> MQVHLTHFELEGLRCLVDKLESLPLHKKCVPTGIEDEDALIADVKILLEELASSDPKLALTGVP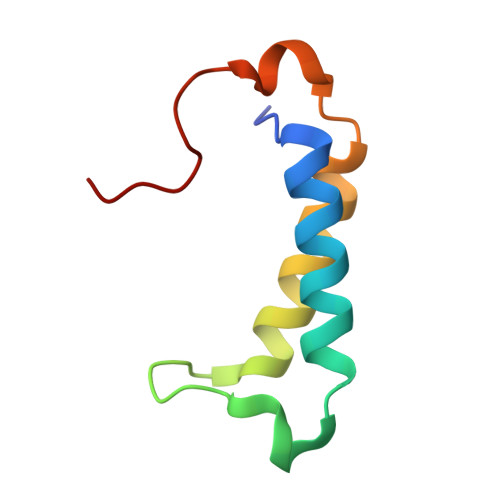IVQWP>MTVKYTDAQIQRLREYGNGTYEQKVFEDLASRDAAFSKEMSVASTDNEKKIKGMIANPSRHGLTQLMNDIADALVAEGFIEVRTPIFISKDALARMTITEDKPLFKQVFWIDEKRALRPMLAPNIFSVGRDLRDHTDGPVKIFEMGSCFRKESHSGMHLEEFTMLNLFDMGPRGDATEVLKNYISVVMKAAGLPDYDLVQEESDVFKETIDVEINGQEVCSAAVGPHYLDAAHDVHEPWSGAGFGLERLLTIREKYSTVKKGGASISYLNGAKINLEHHHHHH[2x]

Transplanting known mutations from a promiscuous Methanosarcina mazei pyrrolysyl‐tRNA synthetase (MmPylRSIFGFF) into a single domain PylRS from Methanomethylophilus alvus (MaPylRSIFGFF) provided a variant with improved efficiency and specificity for 3‐methyl‐L‐histidine (MeHis) incorporation. The MaPylRSIFGFF clone was further characterized using in vitro biochemical assays and x‐ray crystallography. The structure of the C‐terminal catalytic domain of MaPylRS is similar to that of MmPylRS and MbPylRS. MaPylRS lacks an N‐terminal tRNA binding domain that is essential for activity in MmPylRS and MbPylRS, and consequently it is inherently more stable to purification, more amenable to kinetic and structural characterization, and provides opportunities to produce proteins containing ncAAs using cell free expression systems (Gottfried‐Lee et al., 2022; Herring et al., 2007; Jiang & Krzycki, 2012; Seki et al., 2020).

To develop MaPylRS for encoding MeHis, mutations from MmPylRSIFGFF (L305I Y306F L309G C348F Y384F) were mapped onto MaPylRS through alignment of published structures and sequences (Karvan et al., 2007; Seki et al., 2020). The resulting MaPylRSIFGFF (L125I, Y126F, M129G, V168F, and Y206F) variant was evaluated using a GFP production assay and its activity compared to the existing Mm system. Efforts to obtain crystal structures with the amino acid substrate MeHis bound were unsuccessful, and the active site is instead occupied by an exogenous triethylene glycol from the crystallization buffer. As observed in published structures of MaPylRS variants, AMP‐PNP is coordinated by three octahedral magnesium ions, which in turn are coordinated by water and the sidechains of residues E218, and S221 (Gottfried‐Lee et al., 2022). The flexible loop spanning residues 150–160 adopts a similar pose to that observed in AMP‐PNP/ATP bound structures of PylRS homologs. In our structure, the loop harboring residues 199–210 adopts a “closed” conformation, plausibly due to the presence of triethylene glycol positioned in the amino acid binding pocket. Remarkably, in addition to its increased efficiency, MaPylRSIFGFF also displays enhanced specificity compared with MmPylRSIFGFF and has negligible activity toward the histidine analogue 3‐Pyr. Consistent with our in vivo assays, MaPylRSIFGFF can adenylate MeHis with a rate of 0.59 ± 0.05 min−1 at 10 mM substrate concentration. In contrast, no activity is observed using 3‐Pyr as a substrate. Similarly, regioisomeric amino acids 1‐methyl‐histidine and 2‐pyridylalanine are not substrates for MaPylRSIFGFF. These data confirm that the increased selectivity observed with MaPylRSIFGFF arises from the specificity of amino acid adenylation rather than downstream transfer of the activated amino acid to the tRNA.>[4x]GSHMAMSEKPNTQELKQQQ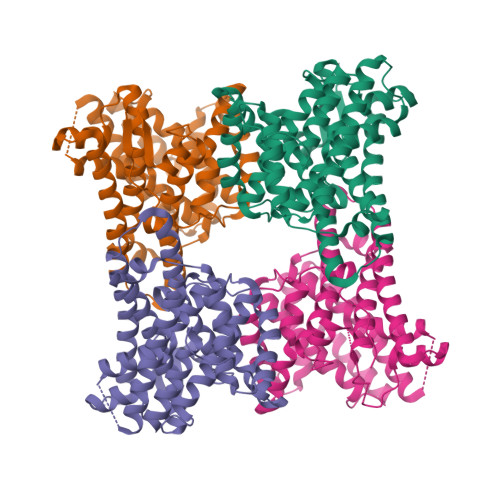LDPKRPPFVRVPDLFGSIMSTKPVVNPNYFAAKARGDRWIARVMNFNKAVAARNSKVDLCFLASMWAPDAPEDRLVMMLDWNHWVFLFDDQFDEGHLKEDPAAAAEEVKQTIAIMGGNAPRYTAESNPIRYVFQQCWDRLKAVSSQEMQQRWIDQHKRYFDQLLVQVDQQVGGENFTRDVEAYMDLRRGTIGVYPAISLSEYGAGVNVPQHVYDHPSLQECMKVSADLVTLVNDVLSYRKDLELGVDHNLMSLLMQRDNLSAQQAVDVIGDMVNECYRRWYLALAELPSYGEKIDYNVMKFVEICRAVAQGNLYWSFQTGRYLGPEGHEVHETGIMYLPPAANLVVA> SGSKYVVIDGEGNEYEFTDLKEAAAKAKELKKKYGFASISVPVEPDEVAVVDGKGNEHTFTDIKKAVEKAKELAKETGFASISVPVEPDEYLVIDGKGNEHKFTDLKEAVAKAKELKKKYGFASVSVPVPAGSG

In pseudocyclic proteins, such as TIM barrels, β barrels, and some helical transmembrane channels, a single subunit is repeated in a cyclic pattern, giving rise to a central cavity that can serve as a pocket for ligand binding or enzymatic activity. Inspired by these proteins, we devised a deep-learning-based approach to broadly exploring the space of closed repeat proteins starting from only a specification of the repeat number and length. Biophysical data for 38 structurally diverse pseudocyclic designs produced in Escherichia coli are consistent with the design models, and the three crystal structures we were able to obtain are very close to the designed structures. The large set of pseudocycles with central binding pockets described here combines the diversity of native protein scaffolds with the stability and robustness of de novo-designed proteins, and our RIF docking and Rosetta design calculations suggest that the designed pseudocycles provide better starting scaffolds for small-molecule binder design than do either native structures or previously designed de novo NTF2s.

a–e, Crystal structures of the five-repeat design E8 (a), two-repeat design H12 (b), and the three-repeat design H10 (c–e) are shown as gray cartoons; the loop, sheets, and helix of the design are shown in dark blue, magenta, and teal, respectively. Central pockets in the designs are shown as gray spheres (a–c). The secondary structure interface (d) and the center-water-mediated hydrogen bond network (e) of the refined crystal structure of design H10 are shown using sticks. The electron density map of the interface and the center hydrogen bond network and water are shown as gray mesh. In d and e, the oxygen, nitrogen, and carbon are colored in red, blue, and magenta, respectively; hydrogen bond networks are shown as yellow dashed lines, and water molecules as red spheres. The approach generates a wide variety of structures strongly encoded by their amino acid sequences (as evaluated with RF and AF2, and further indicated by the close agreement between the crystal structures and design models), with between 2 and 7 repeat units (N), repeat lengths of 15 to 78 (L), and all ɑ-, ɑ/β-, and all β-folds.> XADVAGTSNRDFRGREQRLYNSEQYNYNNSLNGEVSLWVYAYYSDGSVLVRNCNS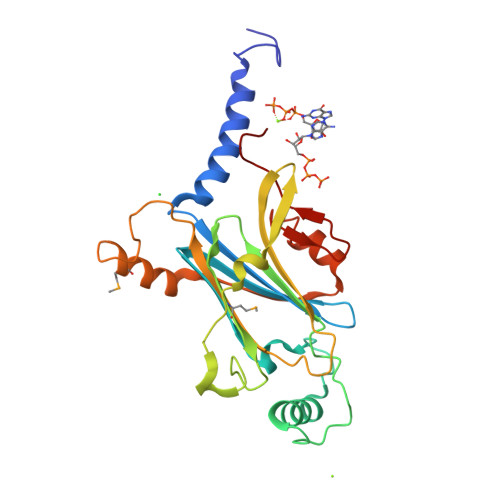QYKVGISECFKSLKEVRVGQNNDPYDEQEVNNGVYYPNGGEPTKFHSNAKPRAIQIIFSPSVNVHTIKMAKGNSVSIPKDYLQRSHPWEATGVKYRKIHVDGEIVGYSHYFELPHEYNSISLSVSGVHKNPSSYNVAAPHNIMDVFQSCDLALKFSNRYWCELELINHYISAYAYPYLDINNHKYGVPLNGRQ> MSQQSSSPTKEDNNSSSPVVPNPDSVPPQLSSPALFYSSSSSQGDIYGRNNSQNLSQGEGNIRAAIGSSPLNFPSSSQRQNSDVFQSQGRQGRIRSSASASGRSRYHSDLRSDRALPTSSSSLGRNGQNRVHMRRNDIHTSDLSSPRRIVDFDTRSGVNTLDTSSSSAPPSEASEPLRIIWGTNVSIQECTTNFRNFLMSFKYKFRKILDEREEFINNTTDEELYYIKQLNEMRELGTSNLNLDARNLLAYKQTEDLYHQLLNYPQEVISIMDQTIKDCMVSLIVDNNLDYDLDEIETKFYKVRPYNVGSCKGMRELNPNDIDKLINLKGLVLRSTPVIPDMKVA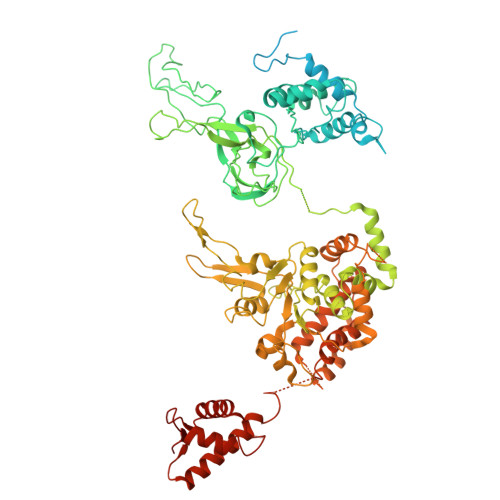FFKCNVCDHTMAVEIDRGVIQEPARCERIDCNEPNSMSLIHNRCSFADKQVIKLQETPDFVPDGQTPHSISLCVYDELVDSCRAGDRIEVTGTFRSIPIRANSRQRVLKSLYKTYVDVVHVKVSSDKRLDVDTSTIEQELMQNKVDHNEVEEVRQITDQDLAKIREVAAREDLYSLLARSIAPSIYELEDVKKGILLQLFGGTNKTFTKGGRYRGDINILLCGDPSTSKSQILQYVHKITPRGVYTSGKGSSAVGLTAYITRDVDTKQLVLESGALVLSDGGVCCIDEFDKMSDSTRSVLHEVMEQQTISIAKAGIITTLNARSSILASANPIGSRYNPNLPVTENIDLPPPLLSRFDLVYLVLDKVDEKNDRELAKHLTNLYLEDKPEHISQDDVLPVEFLTMYISYAKEHIHPIITEAAKTELVRAYVGMRKMGDDSRSDEKRITATTRQLESMIRLAEAHAKMKLKNVVELEDVQEAVRLIRSAIKDYATDPKTGKIDMNLVQTGKSVIQRKLQEDLSREIMNVLKDQASDSMSFNELIKQINEHSQDRVESSDIQEALSRLQQEDKVIVLGEGVRRSVRLNNRV1-(8Z-hexadecenoyl)-sn-glycerol | C19 H36 O4 | 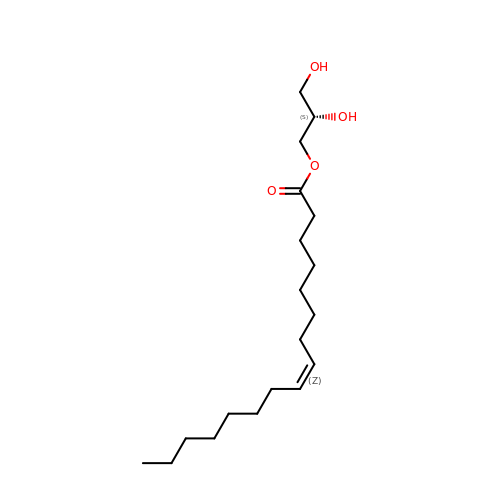CRXZGWVXXGFOLB-GIFJBRJJSA-N>SMDCRTKANPDRTFDLVLKVKCHASENEDPV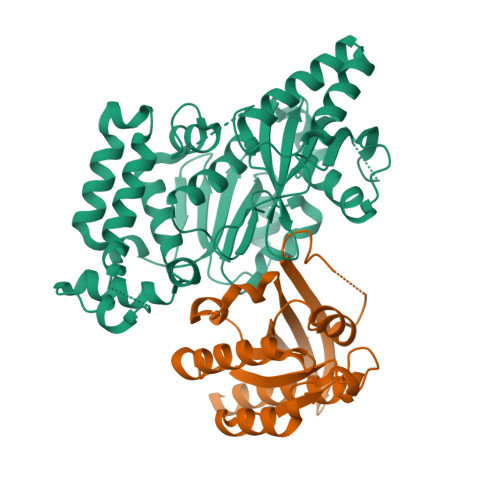VLWKFPEDFGDQEILQSVPKFCFPFDVERVSQNQVGQHFTFVLTDIESKQRFGFCRLTSGGTICLCILSYLPWFEVYYKLLNTLADYLAKELENDLNETLRSLYNHPVPKANTPVNLSVHSYFIAPDVTGLPTIPESRNLTEYFVAVDVNNMLQLYASMLHERRIVIISSKLSTLTACIHGSAALLYPMYWQHIYIPVLPPHLLDYCCAPMPYLIGIHSSLIERVKNKSLEDVVMLNVDTNTLESPFSDLNNLPSDVVSALKNKLKKQSTATGDGVARAFLRAQAALFGSYRDALRYKPGEPITFCEESFVKHRSSVMKQFLETAINLQLFKQFIDGRLAKLNAGRGFSDVFEEEITSGG[2x];>SMARDYDHLFKLLIIGDSGVGKSSLLLRFADNTFSGSYITTIGVDFKIRTVEINGEKVKLQIWDTAGQERFRTITSTYYRGTHGVIVVYDVTSAESFVNVKRWLHEINQNCDDVCRILVGNKNDDPERKVVETEDAYKFAGQMGIQLFETSAKENVNVEEMFNCITELVLRAKKDNLAKQQ[2x]>MGMEFSSHHIRLLQQLDEQRQKDLFCDCHIIVEGQMFKAHRNVLFASSGYFKMLLSQSCRDMGEPITATFDVFSADTFTAILDFVYSGKLPLSGQNVIEVMSAAAYLQMTDVIGVCKMFIKSSLDINEKDRDGFFSLSDKDAGS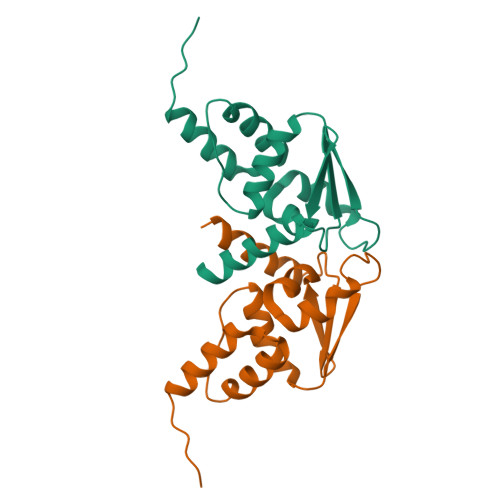NGSGLEHHHHHH[2x]> MSIRYESVENLLTLIKDKKIKPSDVVKDIYDAIEETDPTIKSFLALDKENAIKKAQELDELQAKDQMDGKLFGIPMGIKDNIITNGLETTCASKMLEGFVPIYESTVMEKLHKENAVLIGKLNMDEFAMGGSTETSYFKKTVNPFDHKAVPGGSSGGSAAAVAAGLVPLSLGSDTGGSIRQPAAYCGVVGMKPTYGRVSRFGLVAFASSLDQIGPLTRNVKD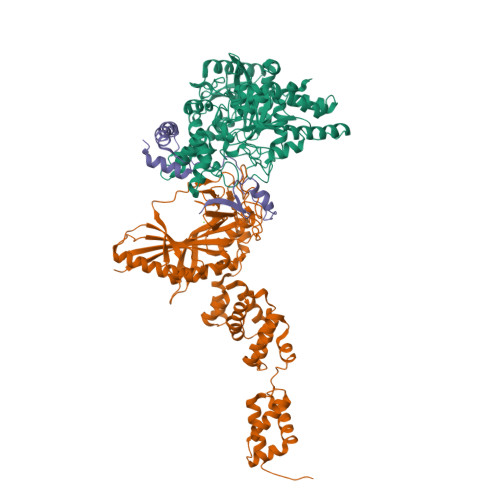NAIVLEAISGADVNDSTSAPVDDVDFTSEIGKDIKGLKVALPKEYLGEGVADDVKEAVQNAVETLKSLGAVVEEVSLPNTKFGIPSYYVIASSEASSNLSRFDGIRYGYHSKEAHSLEELYKMSRSEGFGKEVKRRIFLGTFALSSGYYDAYYKKSQKVRTLIKNDFDKVFENYDVVVGPTAPTTAFNLGEEIDDPLTMYANDLLTTPVNLAGLPGISVPCGQSNGRPIGLQFIGKPFDEKTLYRVAYQYETQYNLHDVYEKL;> MHFETVIGLEVHVELKTDSKMFSPSPAHFGAEPNSNTNVIDLAYPGVLPVVNKRAVDWAMRAAMALNMEIATESKFDRKNYFYPDNPKAYQISQFDQPIGENGYIDIEVDGETKRIGITRLHMEEDAGKSTHKGEYSLVDLNRQGTPLIEIVSEPDIRSPKEAYAYLEKLRSIIQYTGVSDVKMEEGSLRCDANISLRPYGQEKFGTKAELKNLNSFNYVRKGLEYEEKRQEEELLNGGEIGQETRRFDESTGKTILMRVKEGSDDYRYFPEPDIVPLYIDDAWKERVRQTIPELPDERKAKYVNELGLPAYDAHVLTLTKEMSDFFESTIEHGADVKLTSNWLMGGVNEYLNKNQVELLDTKLTPENLAGMIKLIEDGTMSSKIAKKVFPELAAKGGNAKQIMEDNGLVQISDEATLLKFVNEALDNNEQSVEDYKNGKGKAMGFLVGQIMKASKGQANPQLVNQLLKQELDKRLEHHHHHH;> MTKVTREEVEHIANLARLQISPEETEEMANTLESILDFAKQNDSADTEGVEPTYHVLDLQNVLREDKAIKGIPQELALKNAKETEDGQFKVPTIMNEEDA5-[(3,4-dihydroxy-9,10-dioxo-9,10-dihydroanthracene-2-sulfonyl)amino]pentanoic acid | C19 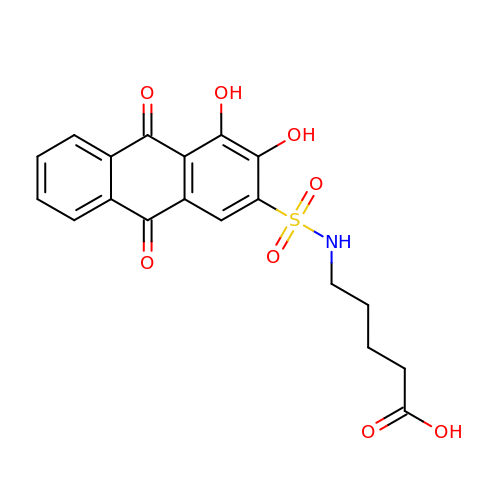H17 N O8 S | QKSBODUPEIWERR-UHFFFAOYSA-N>[6x]MREESWEDHDTIQLTAQRKYLAEVQALETLLTRELSVFLTEPGSKKTNIINRITGKTYALPSTELLRLYEHLEQCRKQGALMYFLERQGTYSGLMLDYDLKLNTNAVPPLEPPALSRLCHRIFVHIKNSSVLPEGSHKIHFFFTLKPEVVQGKYGFHVLIPGLKLAASTKKSIIGSLQHDATVQKILHEQGVTNPESCLDPHSASVPSLLYGSSKLNHKPYQLKTGFELVFDSSDPDYIPIHQ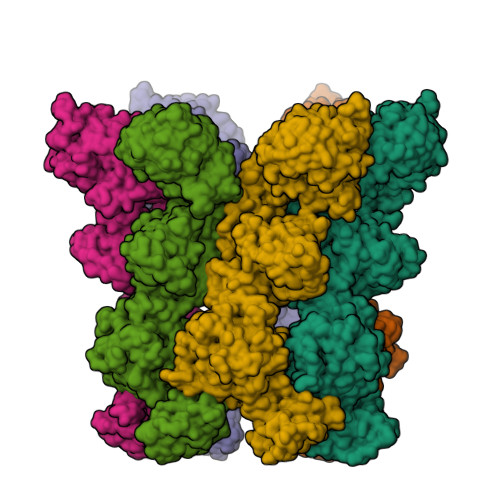IKNLESYNLVSELSLTNEQGSLVRPVYCAADIAAEKEEEIPTEDHSLSILMLHDPEARYLHKILNLLPPEYYVEYPLWSNVVFALANTSANYRPLAEWFSQKCPEKWNTGGKEKLEKLWNDASHHTEKKITKRSIMYWAHKHAPQQYKEIVEQGYFSILAEYVYSYNGMLEHYMIAKVIYAMMGNKFVVDVDSNGKYVWFEFVLPGQPMNQGEIWKWRKEVNPDELHIYISENFSRVMDRITEHIKYHLSQPHESNILNYYKKLLKAFERSKSKIFNDSFKKGVIRQAEFLFRQRSFIQTLDTNPHLLGVGNGVLSIETIPAKLINHFHEHPIHQYTHICYVPFNPENPWTKLLLNALQDIIPELDARLWIMFYLSTAIFRGLKEALMLLWLGGGCNGKTFLMRLVAMVLGDHYASKLNISLLTSCRETAEKPNSAFMRLKGRGYGYFEETNKSEVLNTSRLKEMVNPGDVTARELNQKQESFQMTATMVAASNYNFIIDTTDHGTWRRLRHYRSKVKFCHNPDPSNPYEKKEDPRFIHEYIMDPDCQNAFFSILVYFWEKLQKEYNGQIKKVFCPTIESETEAYRKSQDTLHRFITERVVESPSAETVYNLSEVVTAYAEWYNTNINVKRHIALELSQELENSVLEKYLQWSPNKTRILKGCRILHKFETLQPGESYIGVSTAGTLLNTPICEPKNKWWEWSPNPSAPPEKEASAPTPLEDYKDDDDK> MKKISRKEYVSMYGPTTGDKVRLGDTDLIAEVE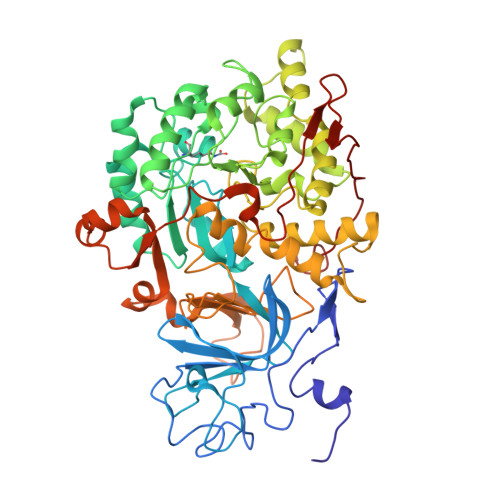HDYTIYGEELKFGGGKTLREGMSQSNNPSKEELDLIITNALIVDYTGIYKADIGIKDGKIAGIGKGGNKDMQDGVKNNLSVGPATEALAGEGLIVTAGGIDTHIHFISPQQIPTAFASGVTTMIGGGTGPADGTNATTITPGRRNLKWMLRAAEEYSMNLGFLAKGNASNDASLADQIEAGAIGFKIHEDWGTTPSAINHALDVADKYDVQVAIHTDTLNEAGCVEDTMAAIAGRTMHTFHTEGAGGGHAPDIIKVAGEHNILPASTNPTIPFTVNTEAEHMDMLMVCHHKDKSIKEDVQFADSRIRPQTIAAEDTLHDMGAFSITSSDSQAMGRVGEVITRTWQTADKNKKEFGRLKEEKGDNDNFRIKRYLSKYTINPAIAHGISEYVGSVEVGKVADLVLWSPAFFGVKPNMIIKGGFIALSQMGDANASIPTPQPVYYREMFAHHGKAKYDANITFVSQAAYDKGIKEELGLERQVLPVKNCRNVTKKDMQFNNTTAHIEVNPETYHVFVDGKEVTSKPANKVSLAQLFSIF> SGRPMFAVAVNEFIRSAGQDSLCGVPDINSSGDFMPLHIIVKEVPKVLPCCRRPKIKRTPYTLNDILDEPCPNQLKSSDLVTFTEPLVSNVKASSSIGLQILKHFDSGAKGSKNFITSASLGTVVKAETIDITKVLAKVRTAKAK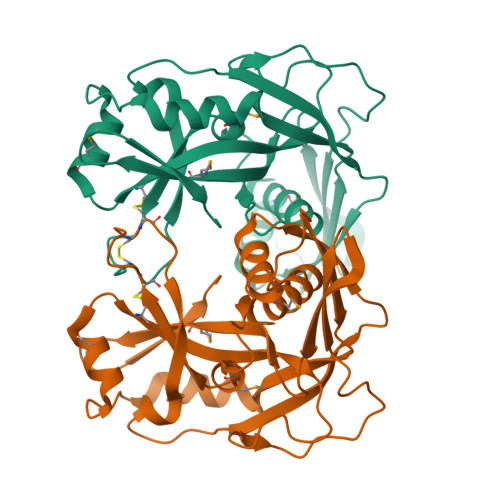VENDLVSRVMKTKRLCLGLVVETACVAAAGKLTEADNWEISGHTNANIGEAVVTATAELDKNLSRKIEIPPGTALAYSFMDLEILEDRSLRVSSSAGA>DYFQGAMGSKPAYSFHVTADGQMQPVPFPPDALIGPGIPRHARQINTLNHGEVVCAVTISNPTRHVYTGGKGCVKV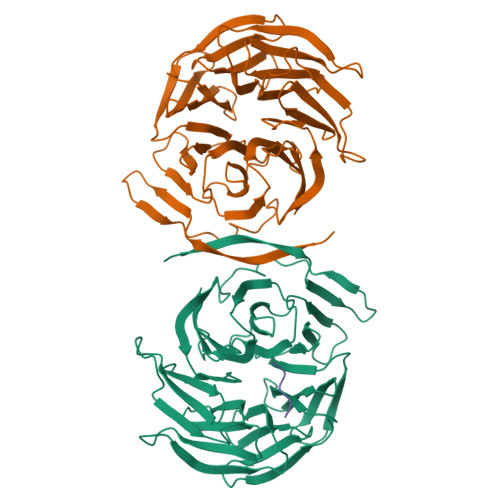WDISHPGNKSPVSQLDCLNRDNYIRSCKLLPDGCTLIVGGEASTLSIWDLAAPTPRIKAELTSSAPACYALAISPDSKVCFSCCSDGNIAVWDLHNQTLVRQFQGHTDGASCIDISNDGTKLWTGGLDNTVRSWDLREGRQLQQHDFTSQIFSLGYCPTGEWLAVGMESSNVEVLHVNKPDKYQLHLHESCVLSLKFAYCGKWFVSTGKDNLLNAWRTPYGASIFQSKESSSVLSCDISVDDKYIVTGSGDKKATVYEVIY[4x];>[2x]MWRPW> GSMSEPFGIVAGALNVAGLFNNCVDCFEYVQLGRPFGRDYERCQLRLDIAKARLSRWGEAVKINDDPRFHSDAPTDKSVQLAKSIVE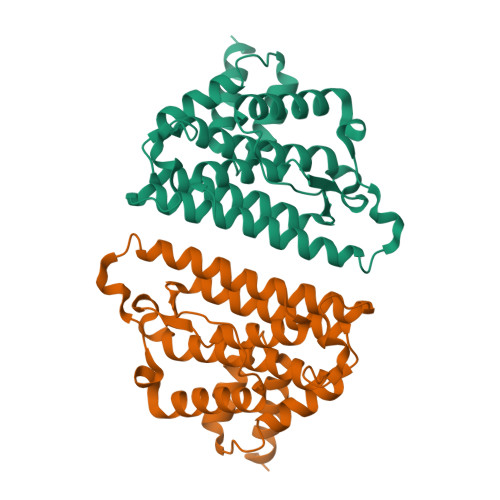EILLLFESAQKTSKRYELVADQQDLVVFEDKDMKPIGRALHRRLNDLVSRRQKQTSLAKKTAWALYDGKSLEKIVDQVARFVDELEKAFPIEAVCHKLAEIEIEEVEDEASLTILKDAAGGIDAAMSDAAAQKIDAIVGRNS> ASMWERV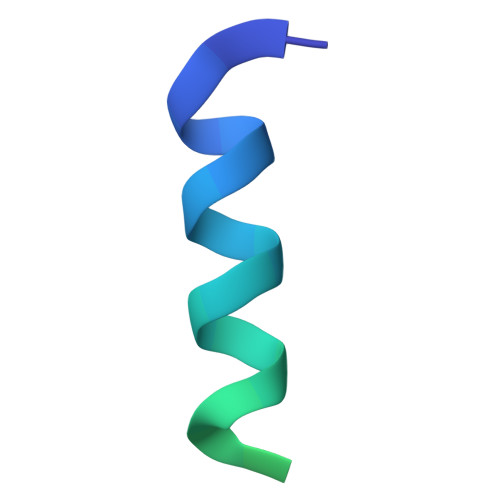KSIIKSSLAMASNVPGPIGIAASGLSGLSALFEGFGF> GAMGSTQQTTHIEALLEKKITEQNELKKRPRRLCTLPNYTKR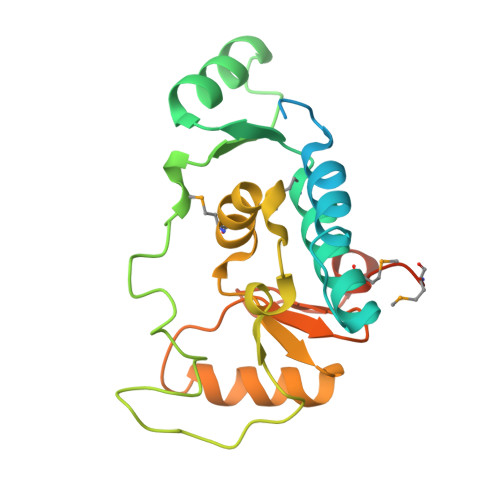SGDILGKIAHLAQIEDDRAAMVISWHLASDMDCVVTLTTDAARAIYDETQGRQQVLPLDSIYRKTLPDWKRPLPHFRNGKLHFKPFGNPVFARDLLTFPDNIEHCETVFGMLLGDTIILDNLDAANHYRKEVVKITHCPTLLTRDGDRIRSNGKFGGLQNKAPPMDKLRGMVFGAPVPKQ The α-amylase from the psychrophilic bacterium Pseudoalteromonas haloplanktis (AHA) is probably the most thoroughly studied cold-adapted enzyme that shows such an anomalous T-optimum, which, in this case, is about 15°C lower than the melting temperature (Tm). Earlier computer simulations of the catalytic reactions of AHA and PPA, based on molecular dynamics (MD) free energy calculations using the empirical valence bond (EVB) method, could directly reproduce the T-optimum of AHA and explain its origin. It was found that a particular binding interaction, between Asp264 of the enzyme and the 2′- and 3′-hydroxyl groups at the −1 position of the oligosaccharide substrate, starts to break precisely at room temperature. Since only the cold-adapted AHA enzyme showed instability of the Asp264-substrate interaction above room temperature, we hypothesized that if its β7-α7 loop conformation could be brought to that found in PPA, then its T-optimum could possibly be raised. In particular, the final model (Chimera 4) that combines 16 mutations in all of the four identified regions above is predicted to almost entirely recover the stable hydrogen bond interaction between Asp264 and the substrate at 25°C, as opposed to the wild-type (WT) enzyme.

To structurally evaluate our computational design, we determined the crystal structures of Chimera 4 in its apo form and in complex with the inhibitor acarbose. The electron density is weak for the two residues Ala271 and Gly272 of the remodeled β7-α7 loop, in both the apo- and holo-structures, so that their backbone conformation cannot be confidently built. There is, however, clear indication from the partial density that the loop conformation is closer to that of PPA than AHA, as intended for Chimera 4. For example, both PPA and Chimera 4 have a well-defined water position that bridges between the carbonyl oxygens of Asn265 and Gly273, and this water molecule would clash with the AHA backbone. Chimera 4, on the other hand, turns out to have a notably larger upshift of the optimum of about 6°C and now shows an activity maximum at around 45°C with this substrate, which is close to that predicted computationally. However, although Chimera 4 has lost a factor of 6 in activity at 25°C, it is now the fastest variant at 50°C, where it is three times faster than AHA and 1.4 times faster than PPA.

> GTPTTFVHLFEWNWQDVAQECEQYLGPKGYAAVQVSPPNEHITGSQWWTRYQPVSYELQSRGGNRAQFIDMVNRCSAVGVDIYVDTLINHMAAGSGTGTAGNSFGNKSFPIYSPQDFHESCTINNSDYGNDRYRVQNCELVGLADLDTASNYVQNTIAAYINDLQAIGVKGFRFDASKHVAASDIQSLMAKVNGSPVVFQEVIDLGGEAIKSSEYLSTGLVTEFKYGAKLGTVFRNGSLAWLSNFGEGWGFMPSSSAVVFVDNHDNQRGHGAGGSSILTFEDGRLYDLANVFMLAYPYGYPRVMSSYDFHGNDWAGGPNVPVHNNGNLECFASNWKCEHRWSYIAGGVDFRNNTADNWAVTNWWDNTNNQISFGRGSSGHMAINKEDSTLTATVQTDMASGQYCNVLKGELSADAKSCSGEVITVNSDGTINLNIGAWDAMAIHKNAKLL> MSRFQSLLCFVLVSLAAVANAAIGPVADLTLTNAAVSPDGFTREAVVVNGITPAPLIAGKKGDRFQLNVIDNLTNHTMLKTTSIHWHGFFQHGTNWADGVSFVNQCPIASGHSFLYDFQVPDQAGTFWYHSHLSTQYCDGLRGPFVVYDPNDPQASLYDIDNDDTVITLADWYHLAAKVGQRFPLGADATLINGLGRTPGTTSADLAVIKVTQGKRYRFRLVSLSCDPNHTFSIDGHTMTIIEADSVNTQPLEVDSIQIFAAQRYSFVLDASQPVDNYWIRANPPFGNVGFAGGINSAILRYDGAPEVEPTTTQTTPTKPLNEADLHPLTPMPVPGRPEPGGVDKPLNMVFNFNGTNFFINNHSFVPPSVPVLLQILSGAQAAQDLVPEGSVYVLPSNASIEISFPATANAPGSPHPFHLHGHTFAVVRSAGSSEYNYDNPVFRDVVSTGTPGDNVTIRFQTNNPGP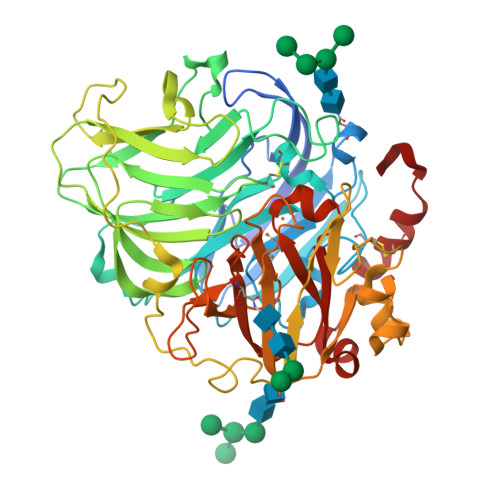WFLHCHIDFHLDAGFAVVMAEDTPDTASVNQVPQSWSDLCPIYDALDPSDL> EPLYENSPEFTPYLETNLGQPTIQSFEQVGTKVNVTVEDERTLVRRNNTFLSLRDVFGKDLIYTLY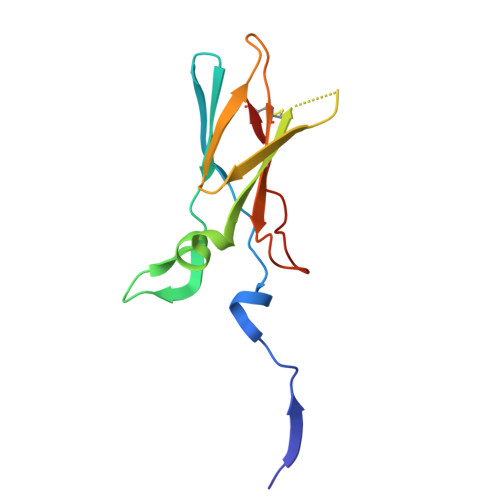YWKSSSSGKKTAKTNTNEFLIDVDKGENYCFSVQAVIPSRTVNRKSTDSPVECM>MAANSLPTNVASPVQTTTPTTDKRSIGFIDRQLGTNPAELPPLPYGYDALEKAIDAETMKLHHDKHHAAYVNNLNNALKKHPELQNSSVEALLRDLNSVPEDIRTTVRNNGGGHLNHTIFWQIMSPDGGGQPTGDIAQEINQTFGSFEEFKKQFNQAGGDRFGSGWVWLVRNPQGQLQVVSTPNQDNPIM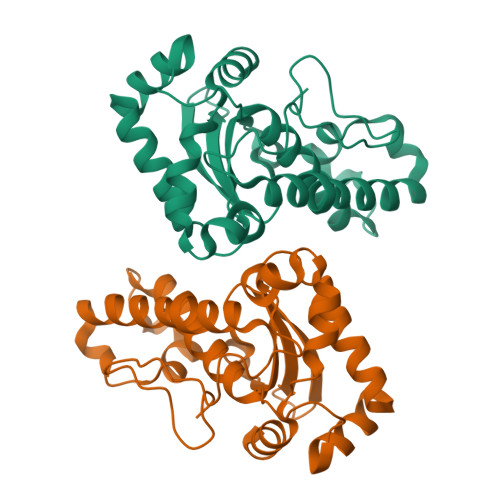EGSYPIMGNDVWEHAYYLRYQNRRPEYLNNWWNVVNWSEINRRTQASRQSNSHHHHHH[2x]>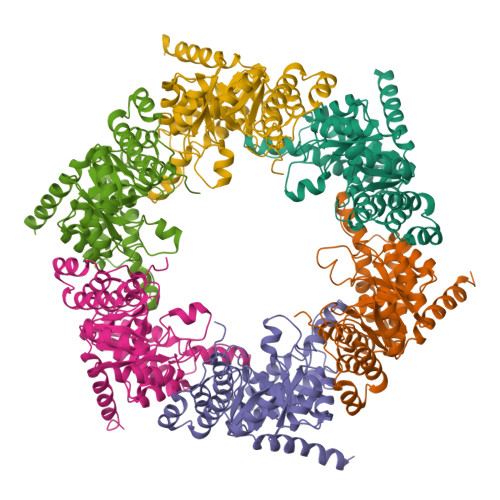MDKLKIIMEKGTERLKRGFAKMVKGGVIMDVTNAEQARIAEEAGAVAVMALHKVPADIRKAGGVARMAPVEKIQEIMDAVTIPVMAKCRIGHEAEARILEALGVDMIDESEVLTPADPFFHIYKKKFTAPFVCGARNLGEAVRRIWEGAAMIRTKGEAGTGNIIEAVRHVRLVNENIRLIQRMTDEEIYGVAEKFAEPYLRLAFSVKEISGLPKRVLENEPIYEGFTYREIVEDIYKILLEIKKLGRLPVVNFAAGGVATPADAALMMAMGMDGVFVGSGIFKSSNPPKMARAIVEAVNHWDEPDVLAEISREIGEPMRGQAIEELQVRMEERGI[6x]> LQ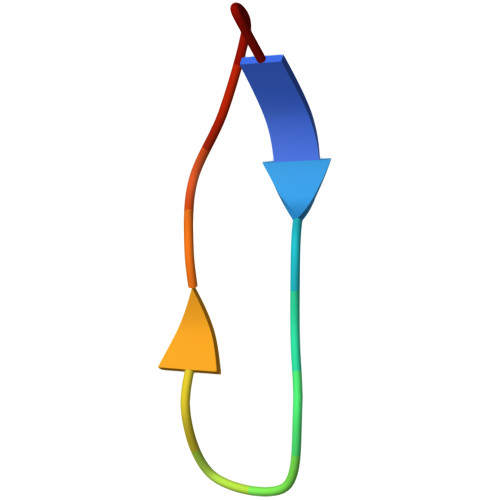LTLGNSTITTQE> SQDPYFKIANWTNEHDDFKKAEMRMDEKHRKKVDKVMKEWGDLETRYNEQKAKDPKGAEKFKSQMNARFQKTVSSLEEEHKRMRKEIEAVHEERVQAMLNEKKRDATHDYRQALATHVNKPNKHSVLQSLKAYIRAEEKDRMHT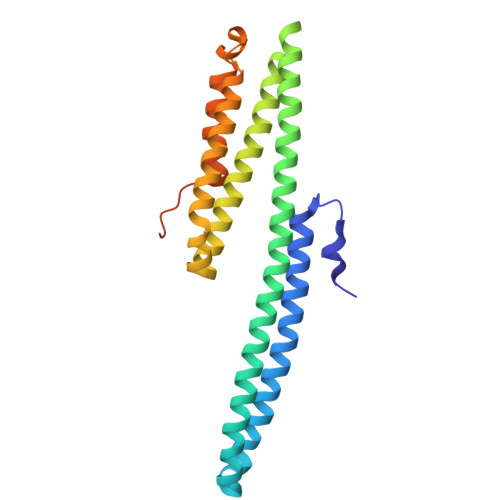LNRYRHLLKADSKEAAAYKPTVIHRLRYIDLRINGTLAMLRDFPDLEKYVRPIAVTYWKDYRDEVSPDISVEDSELTPIIHDDEFSKNAKLDVKA> MKFRLPQYAYIIGTRGNVKDHMRRMLVEQHEVDRSVFKAVTTDKSVP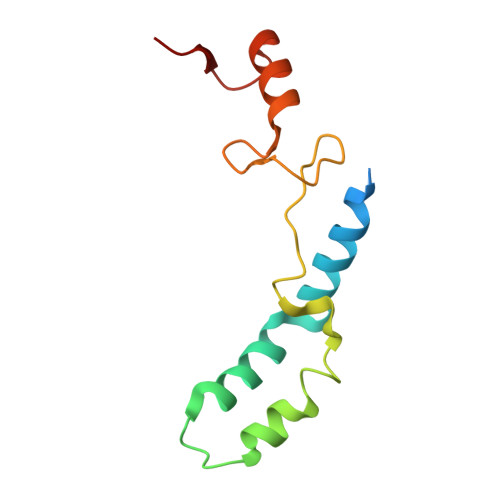LEHRLQVQRLFETEVPRDSAANRVVNRCVLTGRARGVHRFARLSRIMIRQLAHSGFLPGVSKASW>[4x]GSESSRSAMMYIQELRSGLRDMHLLSCLESLRVSLNNNPVSWVQTFGAEGLASLLDILKRLHDEKEETSGNYDSRNQHEIIRCLKAFMNNKFGIKTMLETEEGILLLVRAMDPAVPNMMIDAAKLLSALCILPQPEDMNERVLEAMTERAEMDEVERFQPLLDGLKSGTSIALKVGCLQLINALITPAEELDFRVHIRSELMRLGLHQVLQELREIENEDMKVQLCVFDEQGDEDFFDLKGRLDDIRMEMDDFGEVFQIILNTVKDSKAEPHFLSILQHLLLVRNDYEARPQYYKLIEECVSQIVLHKNGTDPDFKCRHLQIDIERLVDQ;>GSFGFGVPAAPVLPFGL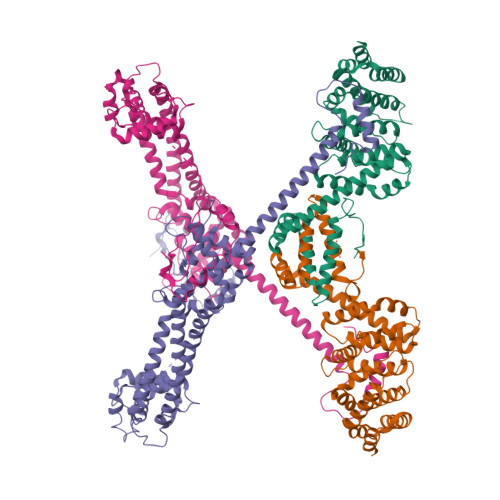TPKKVYKPEVQLRRPNWSKFVAEDLSQDCFWTKVKEDRFENNELFAKLTLAFSAQTKTSKAKKDQEGGEEKKSVQKKKVKELKVLDSKTAQNLSIFLGSFRMPYQEIKNVILEVNEAVLTESMIQNLIKQMPEPEQLKMLSELKEEYDDLAESEQFGVVMGTVPRLRPRLNAILFKLQFSEQVENIKPEIVSVTAACEELRKSENFSSLLELTLLVGNYMNAGSRNAGAFGFNISFLCKLRDTKSADQKMTLLHFLAELCENDHPEVLKFPDELAHVEKASRVSAENLQKSLDQMKKQIADVERDVQNFPAATDEKDKFVEKMTSFVKDAQEQYNKLRMMHSNMETLYKELGDYFVFDPKKLSVEEFFMDLHNFRNMFLQAVKENQKRRETEEKMRRAKLAKEKAEKERLEKQQKREQLIDMNAEGDETGVMDSLLEALQSGAAFRRKRG[4x]> MTIDDSNRLLMDVDQFDFLDDGTAQLSNNKTDEEEQLYKRDPVSGAILVPMTVNDQPIEKNGDKMPLK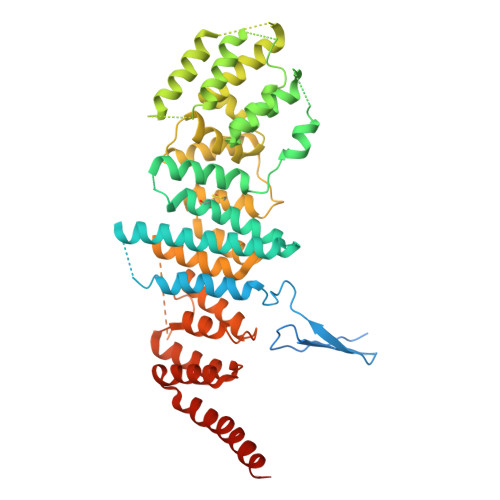FKLGPLSYQNMAFITAKDKYKLYPVRIPRLDTSKEFSAYVSGLFEIYRDLGDDRVFNVPTIGVVNSNFAKEHNATVNLAMEAILNELEVFIGRVKDQDGRVNRFYELEESLTVLNCLRTMYFILDGQDVEENRSEFIESLLNWINRSDGEPDEEYIEQVFSVKDSTAGKKVFETQYFWKLLNQLVLRGLLSQAIGCIERSDLLPYLSDTCAVSFDAVSDSIELLKQYPKDSSSTFREWKNLVLKLSQAFGSSATDISGELRDYIEDFLLVIGGNQRKILQYSRTWYESFCGFLLYYIPSLELSAEYLQMSLEANVVDITNDWEQPCVDIISGKIHSILPVMESLDSCTAAFTAMICEAKGLIENIFEGEKNSDDYSNEDNEMLEDLFSYRNGMASYMLNSFAFELCSLGDKELWPVAIGLIALSATGTRSAKKMVIAELLPHYPFVTNDDIEWMLSICVEWRLPEIAKEIYTTLGNQMLSAHNIIESIANFSRAGK> KETAAAKFERQHMDSSTSAASSSNYCNQMMKSRNLTKDRCKPVNTFVHESLADVQAACSQKNVACKNGQTNCYQSYSTMSITDCRETGSSKYPNCAYKTTQANKHI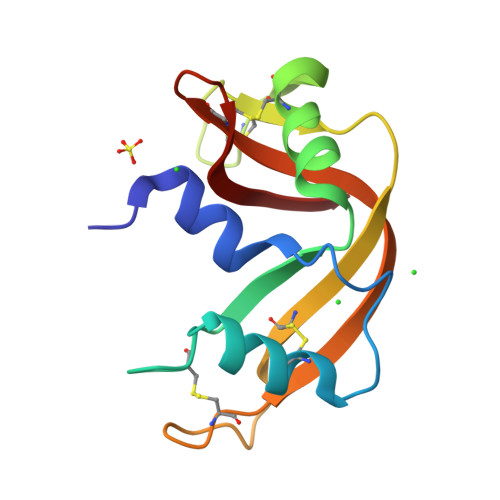IVACEGNPYVPVHFDASV2-[4-[4-cyclopentyl-3-[(1~{S},2~{R})-2-pyridin-2-ylcyclopropyl]phenyl]phenyl]sulfonylethanol 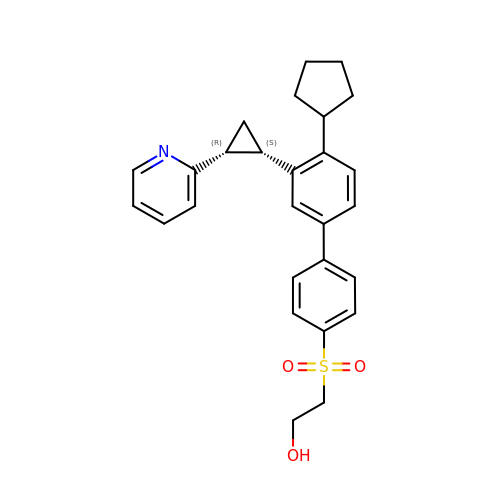| C27 H29 N O3 S | SQNBJZZENOHHKX-CLJLJLNGSA-N>SDAERDALNIETAIKTKGVDEVTIVNILTNRSNAQRQDIAFAYQRRTKKELASALKSALSGHLETVILGLLKTPAQYDASELKASMKGLGTDEDSLIEIICSRTNQELQEINRVYKEMYKTDLEKDIISDTSGDFRKLMVALAKGRRAEDGSVIDYELIDQDARDLYDAGVKRKGTDVPKWISIMTERSVPHLQKVFDRYKSYSPYDMLESIRKEVKGDLENAFLNLVQCIQNKPLYFADRLYDSMKGKGTRDKVLIRIMASRSEVDMLKIRSEFKRKYGKSLYYYIQQDTKGDYQKALLYLCGGDD[2x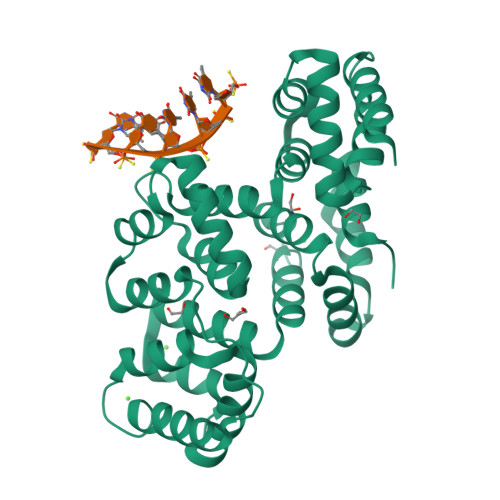]3-(4-nitrophenyl)-1H-pyrazole | C9 H7 N3 O2 | 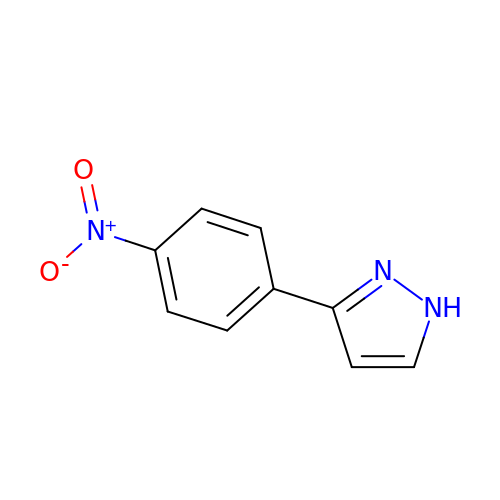IPIYADCDDIUVPS-UHFFFAOYSA-N> GPLGSPEFPHPLQDSWSYYLFQFRKALDWDECLEKVATFSTIEDFWSVLTHTVRPREITYGKDLYMFKSDIMPKWEDPKNENGGRWLINVTARQDVDF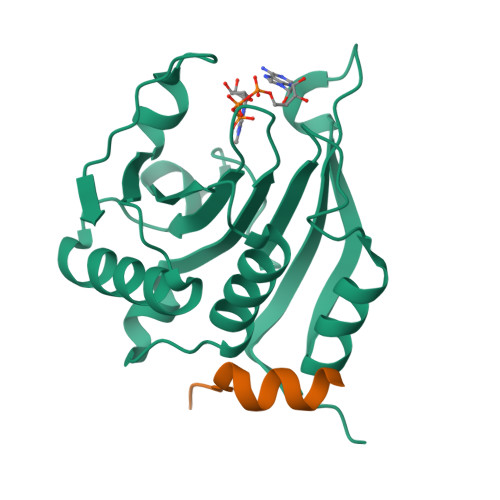LWDELLMLLIGSDWDTDEEDRQICGAVFQPRSRGSKLSVWLTSDNEEETILSIGRRIKERLELEDTIYFQPVSDQRSQTRGSDICTGKYEI;> SGSGRIIYDRKFLMECRNSPV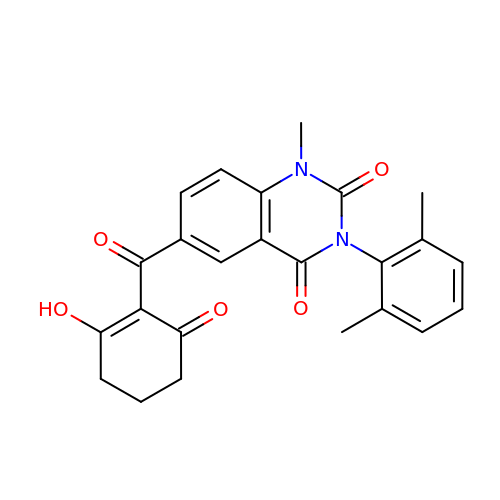3-(2,6-dimethylphenyl)-1-methyl-6-(2-oxidanyl-6-oxidanylidene-cyclohexen-1-yl)carbonyl-quinazoline-2,4-dione | C24 H22 N2 O5 | IFHRYUOSJUERAZ-UHFFFAOYSA-N> QKIGILGAMREEITPILELFGVDFEEIPLGGNVFHKGV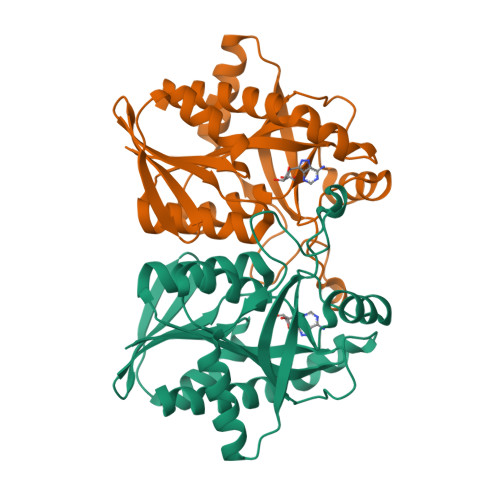YHNKEIIVAYSKIGKVHSTLTTTSMILAFGVQKVLFSGVAGSLVKDLKINDLLVATQLVQHDVDLSAFDHPLGFIPESAIFIETSGSLNALAKKIANEQHIALKEGVIASGDQFVHSKERKEFLVSEFKASAVEMEGASVAFVCQKFGVPCCVLRSISDNADEKAGMSFDEFLEKSAHTSAKFLKSMVDEL> PVNLIFCYTILQMKVAERIMAQHPGERFYVVLMSENNNEKYDYYFNQIKDKAEWAYFFHLPYGLNKSFNFIPTMAELKVKAMLLPKVKRIYLASLEKVSIAAFLSTYPDAE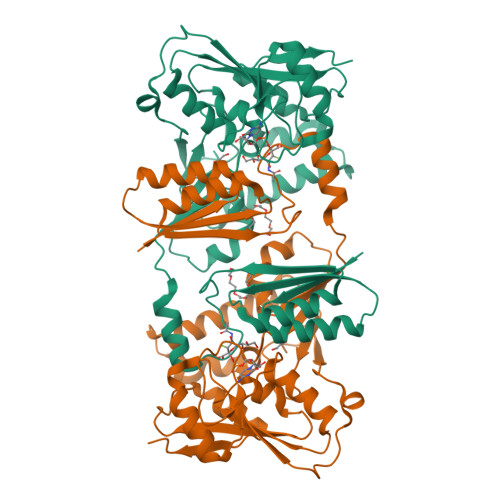IKTFDDGTINLIQSSSYLGDEFSVNGTIKRNFARMMIGDWSIAKTRNASDEHYTIFKGLKNIMDDGRRKMTYLPLFDASELKAGDETGGTVRILLGSPDKEMKEISEKAAKNFNIQYVAPHPRQTYGLSGVTTLNSPYVIEDYILREIKKNPHTRYEIYTFFSGAALTMKDFPNVHVYALKPASLPEDYWLKPVYALFTQSGIPILTFDDKLVPR>[3x]GMIQIDALPAFNDNYIWLLQDATSRRCAVVDPGDAKPVEAWLAAHPDWRLSDILVT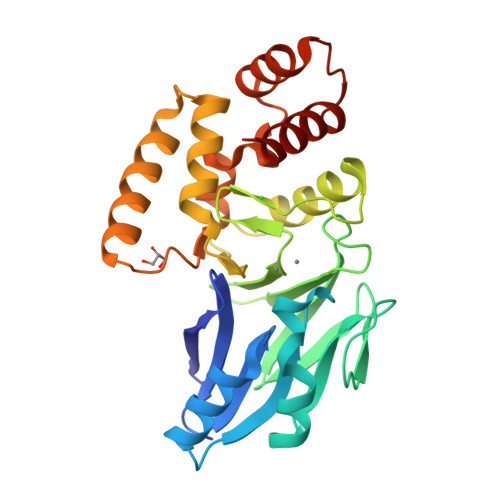HHHHDHVGGVAALKELTGARVLGPANEKIPARDLALEDGERVEVLGLVFEIFHVPGHTLGHIAYYHPAETPLLFCGDTLFAAGCGRLFEGTPAQMHHSLARLAALPANTRVYCTHEYTLSNLRFALAVEPDNAALRERFEEATRLRERDRITLPSEISLELSTNPFLRVSENSVKKKADQRSGQQNRTPEEVFAVLRAWKDQF>[2x]MAAHRPVEWVQAVVSRFDEQLPIKTGQQNTHTKVSTEHNKECLINISKYKFSLVISGLTTILKNVNNMRIFGEAAEKNLYLSQLIILDTLEKCLAGQPKDTMRLDETMLVKQLLPEICHFLHTCREGNQHAAELRNSASGVLFSLSCNNFNAVFSRISTRLQELTVCSEDNVDVHDIELLQYINVDCAKLKRLLKETAFKFKALKKVAQLAVINSLEKAFWNWVENYPDEFTKLYQIPQTDMAECAEKLFDLVDGFAESTKRKAAVWPLQIILLILCPEIIQDISKDVVDENNMNKKLFLDSLRKALAGHGGSRQLTESAAIACVKLCKASTYINWEDNSVIFLLVQSMVVDLKNLLFNPSKPFSRGSQPADVDLMIDCLVSCFRISPHNNQHFKICLAQNSPSTFHYVLVNSLHRIITNSALDWWPKIDAVYCHSVELRNMFGETLHKAVQGCGAHPAIRMAPSLTFKEKVTSLKFKEKPTDLETRSYKYLLLSMVKLIHADPKLLLCNPRKQGPETQGSTAELITGLVQLVPQSHMPEIAQEAMEALLVLHQLDSIDLWNPDAPVETFWEISSQMLFYICKKLTSHQMLSSTEILKWLREILICRNKFLLKNKQADRSSCHFLLFYGVGCDIPSSGNTSQMSMDHEELLRTPGASLRKGKGNSSMDSAAGCSGTPPICRQAQTKLEVALYMFLWNPDTEAVLVAMSCFRHLCEEADIRCGVDEVSVHNLLPNYNTFMEFASVSNMMSTGRAALQKRVMALLRRIEHPTAGNTEAWEDTHAKWEQATKLILNYPKAKMEDGQAAESLHKTIVKRRMSHVSGGGSIDLSDTDSLQEWINMTGFLCALGGVCLQQRSNSGLATYSPPMGPVSERKGSMISVMSSEGNADTPVSKFMDRLLSLMVCNHEKVGLQIRTNVKDLVGLELSPALYPMLFNKLKNTISKFFDSQGQVLLTDTNTQFVEQTIAIMKNLLDNHTEGSSEHLGQASIETMMLNLVRYVRVLGNMVHAIQIKTKLCQLVEVMMARRDDLSFCQEMKFRNKMVEYLTDWVM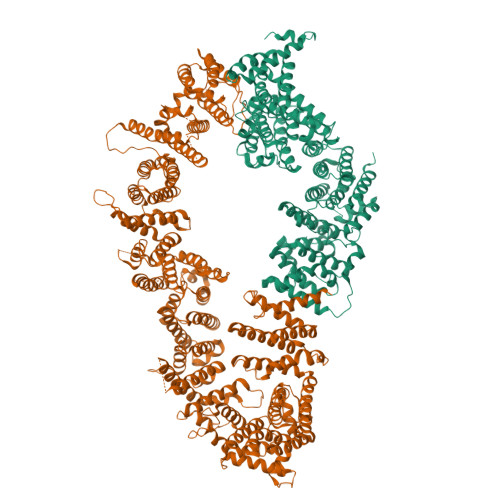GTSNQAADDDVKCLTRDLDQASMEAVVSLLAGLPLQPEEGDGVELMEAKSQLFLKYFTLFMNLLNDCSEVEDESAQTGGRKRGMSRRLASLRHCTVLAMSNLLNANVDSGLMHSIGLGYHKDLQTRATFMEVLTKILQQGTEFDTLAETVLADRFERLVELVTMMGDQGELPIAMALANVVPCSQWDELARVLVTLFDSRHLLYQLLWNMFSKEVELADSMQTLFRGNSLASKIMTFCFKVYGATYLQKLLDPLLRIVITSSDWQHVSFEVDPTRLEPSESLEENQRNLLQMTEKFFHAIISSSSEFPPQLRSVCHCLYQATCHSLLNKATVKEKKENKKSVVSQRFPQNSIGAVGSAMFLRFINPAIVSPYEAGILDKKPPPRIERGLKLMSKILQSIANHVLFTKEEHMRPFNDFVKSNFDAARRFFLDIASDCPTSDAVNHSLSFISDGNVLALHRLLWNNQEKIGQYLSSNRDHKAVGRRPFDKMATLLAYLGPPEHKPVADTHWSSLNLTSSKFEEFMTRHQVHEKEEFKALKTLSIFYQAGTSKAGNPIFYYVARRFKTGQINGDLLIYHVLLTLKPYYAKPYEIVVDLTHTGPSNRFKTDFLSKWFVVFPGFAYDNVSAVYIYNCNSWVREYTKYHERLLTGLKGSKRLVFIDCPGKLAEHIEHEQQKLPAATLALEEDLKVFHNALKLAHKDTKVSIKVGSTAVQVTSAERTKVLGQSVFLNDIYYASEIEEICLVDENQFTLTIANQGTPLTFMHQECEAIVQSIIHIRTRWELSQPDSIPQHTKIRPKDVPGTLLNIALLNLGSSDPSLRSAAYNLLCALTCTFNLKIEGQLLETSGLCIPANNTLFIVSISKTLAANEPHLTLEFLEECISGFSKSSIELKHLCLEYMTPWLSNLVRFCKHNDDAKRQRVTAILDKLITMTINEKQMYPSIQAKIWGSLGQITDLLDVVLDSFIKTSATGGLGSIKAEVMADTAVALASGNVKLVSSKVIGRMCKIIDKTCLSPTPTLEQHLMWDDIAILARYMLMLSFNNSLDVAAHLPYLFHVVTFLVATGPLSLRASTHGLVINIIHSLCTCSQLHFSEETKQVLRLSLTEFSLPKFYLLFGISKVKSAAVIAFRSSYRDRSFSPGSYERETFALTSLETVTEALLEIMEACMRDIPTCKWLDQWTELAQRFAFQYNPSLQPRALVVFGCISKRVSHGQIKQIIRILSKALESCLKGPDTYNSQVLIEATVIALTKLQPLLNKDSPLHKALFWVAVAVLQLDEVNLYSAGTALLEQNLHTLDSLRIFNDKSPEEVFMAIRNPLEWHCKQMDHFVGLNFNSNFNFALVGHLLKGYRHPSPAIVARTVRILHTLLTLVNKHRNCDKFEVNTQSVAYLAALLTVSEEVRSRCSLKHRKSLLLTDISMENVPMDTYPIHHGDPSYRTLKETQPWSSPKGSEGYLAATYPTVGQTSPRARKSMSLDMGQPSQANTKKLLGTRKSFDHLISDTKAPKRQEMESGITTPPKMRRVAETDYEMETQRISSSQQHPHLRKVSVSESNVLLDEEVLTDPKIQALLLTVLATLVKYTTDEFDQRILYEYLAEASVVFPKVFPVVHNLLDSKINTLLSLCQDPNLLNPIHGIVQSVVYHEESPPQYQTSYLQSFGFNGLWRFAGPFSKQTQIPDYAELIVKFLDALIDTYLPGIDEETSEESLLTPTSPYPPALQSQLSITANLNLSNSMTSLATSQHSPGIDKENVELSPTTGHCNSGRTRHGSASQVQKQRSAGSFKRNSIKKIV> GVMTVPNTPQ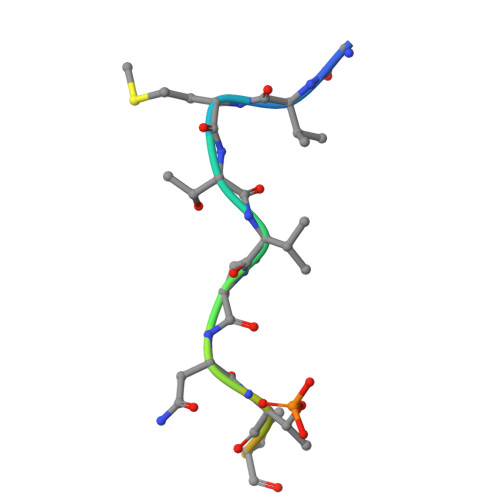KPNLQ N-[(1S)-2-{[(1R)-2-(benzyloxy)-1-cyano-1-methylethyl]amino}-1-(cyclohexylmethyl)-2-oxoethyl]morpholine-4-carboxamide | C25 H36 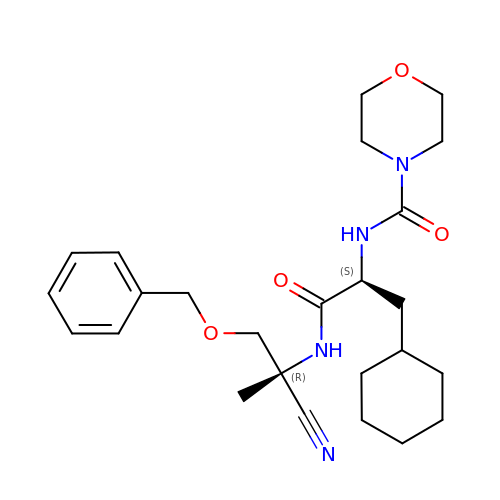N4 O4 | MQWUTQCRGGBPBT-WIOPSUGQSA-N4'-[(1R)-1-amino-2-(2,5-difluorophenyl)ethyl]biphenyl-3-carboxamide 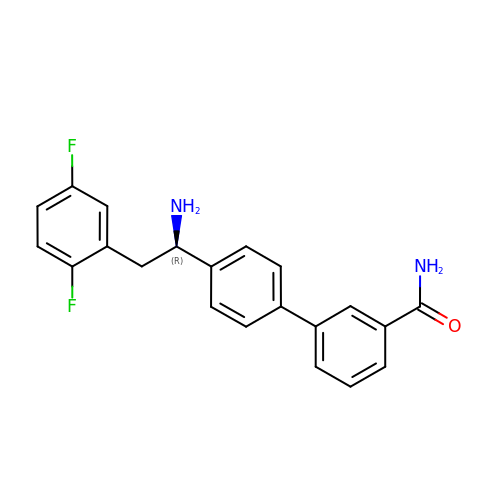| C21 H18 F2 N2 O | JYKFWUXBFJJDTP-HXUWFJFHSA-N>[2x]MEPLDELDLLLLEEDGGAEAVPRVELLRKKADALFPETVLSRGVDNRYLVLAVETSQNERGAEEKRLHVTASQDREHEVLCILRNGWSSVPVEPGDIVHLEGDCTSEPWIIDDDFGYFILYPDMMISGTSVASSIRCLRRAVLSETFRGSDPATRQMLIGTILHEVFQKAISESFAPERLQELALQTLREVRHLKEMYRLNLSQDEILCEVEEYLPSFSKWAEDFMRKGPSSEFPQMQLSLPSDGSNRSSPCNIEVVKSLDIEESIWSPRFGLKGKIDVTVGVKIHRDCKMKYKVMPLELKTGKESNSIEHRSQVVLYTLLSQERREDPEAGWLLYLKTGQMYPVPANHLDKRELLKLRNWLAASLLHRVSRAAPGEEARLSALPQIIEEEKTCKYCSQIGNCALYSRAVEEQGDDASIPEAMLSKIQEETRHLQLAHLKYFSLWCLMLTLESQSKDNRKTHQSIWLTPASELEESGNCVGNLVRTEPVSRVCDGQYLHNFQRKNGPMPATNLMAGDRIILSGEERKLFALSKGYVKKMNKAAVTCLLDRNLSTLPATTVFRLDREERHGDISTPLGNLSKLMESTDPSKRLRELIIDFREPQFIAYLSSVLPHDAKDTVANILKGLNKPQRQAMKRVLLSKDYTLIVGMPGTGKTTTICALVRILSACGFSVLLTSYTHSAVDNILLKLAKFKVGFLRLGQSHKVHPDIQKFTEEEICRSRSIASLAHLEELYNSHPIVATTCMGINHPIFSRKTFDFCIVDEASQISQPVCLGPLFFSRRFVLVGDHQQLPPLVVNREARALGMSESLFKRLERNESAVVQLTVQYRMNRKIMSLSNKLTYAGKLECGSDRVANAVLALPNLKDARLSLQLYADYSDSPWLAGVLEPDNPVCFLNTDKVPAPEQVENGGVSNVTEARLIVFLTSTFIKAGCSPSDIGVIAPYRQQLRIISDLLARSSVGMVEVNTVDKYQGRDKSLILVSFVRSNEDGTLGELLKDWRRLNVALTRAKHKLILLGSVSSLKRFPPLGTLFDHLNAEQLILDLPSREHESLSHIL

Dna2 has nuclease and helicase activities and plays key roles in maintaining genomic integrity. It is involved in the nucleolytic processing of 5’ flaps during Okazaki fragment maturation, of DNA double-strand breaks (DSBs) during homologous-recombination mediated repair, and of stalled replication forks in the intra-S-phase checkpoint. Dna2 contains a PD-(D/E)XK superfamily nuclease motif and a 5’ to 3’ helicase domain. It is a ssDNA endonuclease that requires a free end for cleavage, and does not cleave dsDNA, single-stranded gaps, D-loops or RNA.

The structure consists of a ∼310 residue domain that contains the PD-(D/E)XK nuclease motif, followed by a ∼450 residue, C-terminal helicase domain that has two RecA-like folds characteristic of the SF1 helicase subfamily (domains 1A and 2A). In addition, the structure reveals an OB (oligonucleotide/oligosaccharide-binding) fold domain N-terminal to the nuclease domain, and a β barrel domain that occurs between the nuclease and helicase domains and which is held in place by a stalk of two long alpha helices. The base of the cylinder is formed by the nuclease domain, which adopts a doughnut-like structure with the active site embedded in the central tunnel. The β barrel and helicase 1A domains pack on top of the nuclease doughnut and extend the cylinder and central tunnel. The helicase 2A domain, which packs with the 1A domain as in the ADP states of other SF1 helicase structures, hangs over the tunnel opening at the top of the cylinder. The OB domain decorates the exterior of the nuclease domain, and is uninvolved in DNA binding. In particular, both proteins have a β–α–α N-terminal extension and an α–α C-terminal extension that are stapled together by the iron-sulfur cluster.> 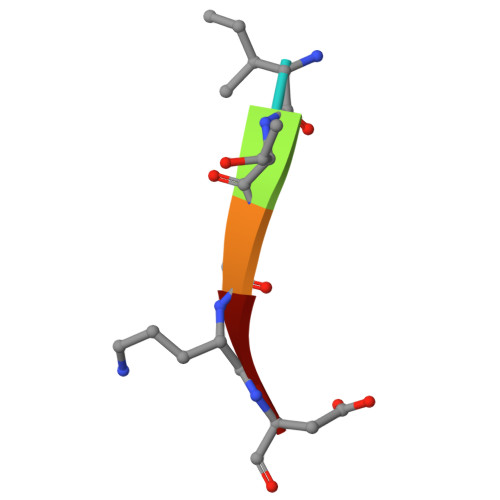ITVAD C16 alpha-bromoamide | C27 H53 Br N3 O8 P | 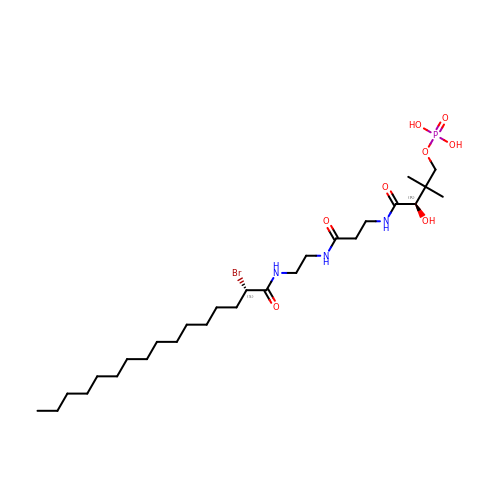WRZPJKRMVZRMQR-UPVQGACJSA-N>[2x]MRRHGFSLLELLLASVLMGSLLLVVLALENSSATLRERERARGRLADELSLTATVLARELYTVGYRLTGQALVLSPSSQGDGVQGWFLCEAGMEEICGESMGEVRGTGYEVNQGALRWGACKGEGCAPLPNNPVLGGDEVQVEAFRVAYLEGGTWKRQAQAVNLRPEGASPKVSALALYLLASVPVRGGAPAFTPGSTLSYPPGLTSSLLELPGAPNDGRLRAEKLWIVQTPNLAR

Type IV pili (T4P)1 are long, surface-exposed filaments which extend from the surfaces of bacterial cells. T4P are composed of both major and minor pilin components, although major pilins comprise the majority of the pilin subunits within each fibre. We identified a cluster of type IV pilin-like genes within the T. thermophilus HB8 genome, using the program PilFind. Three of the remaining six, TTHA1218, TTHA1219 and TTHA1222, yielded crystals of truncated forms which enabled us to solve their structures (designated here as Tt121836-123, Tt121933-236 and Tt122238-123).

Tt121933-236 crystallized in two different crystal forms; the higher resolution form, at 1.85 Å resolution in spacegroup P21, has four molecules in the asymmetric unit, arranged as a dimer of dimers. The second crystal form, in spacegroup C2, has a dimer in the asymmetric unit; crucially, the interface between the A and B chain dimer is preserved in this crystal form, providing further evidence that this dimer is not a crystallization artifact. The monomer-monomer interface is dominated by the helix-helix interaction across the non-crystallographic 2-fold symmetry axis. Tt121933-236 forms a more complex fold topology than XcpW and the related T2SS pseudopilins, with two main differences. First, two additional β-strands, β8 and β9, are inserted into the variable β-sheet, which extend this structural feature into the same spatial location occupied by the short α2 helix in XcpW. Second, Tt121933-236 contains a long loop, from residue 184 in β10 to 221 in β11, which folds back over the external surface of the conserved sheet (marked in orange in Figs4c & d). This has the effect of covering the external face of the conserved sheet. The hydrophobic properties of this face of the conserved β-sheet have been remarked on previously for XcpW, with the suggestion that it could serve as the site for packing of another pseudopilin. Interestingly, addition of this loop in Tt121933-236 preserves this feature of a hydrophobic surface, as apparent from the calculated electrostatic surface (see far right of Fig.4d). Tt121933-236 is also stabilized by two disulphide bonds, between β2/β3, and β4/β5; both lie within the variable β-sheet. Our results show that TTHA1218 and TTHA1219 are closer in structure to T2SS pseudopilins than to other type IV pilins for which structures are currently available.> AASGSALIFDEEMSRYKLLWTDPACEIEVPERLTVSYEALRTHGLAQRCKAVPVRQATEQEILLAHSEEYLEAVKQTPGMNVEELMAFSKKYNDVYFHQNIYHCAKLAAGATLQLVDSVMKREVRNGMALVRPPGHHSQRSAANGFCVFNNVAFAALYAKKNYNLNRILIVDWDVHHGQGIQYCFEEDPSVLYFSWHRYEHQSFWPNLPESDYSSVGKGKGSGFNINLPWNKVGMTNSDYLAAFFHVLLPVAYEFDPELVIVSAGFDSAIGDPEGEMCALPEIFAHLTHLLMPLAAGKMCVVLEGGFNLTSLGQSVCQTVHSLLGDPTPRISGLGTACDSALESIQNVRNVQSSYWSSFKHLAQSETNPKRPRLDATNGGPKESSEPASESNPKKTAQDIVWPEPLKRMPASVRTVVVPPPGVELTLPKNCQHSGDISESTAKEVQRIRDKHFHDLTDQNILRSLGNIISVLDRMMRS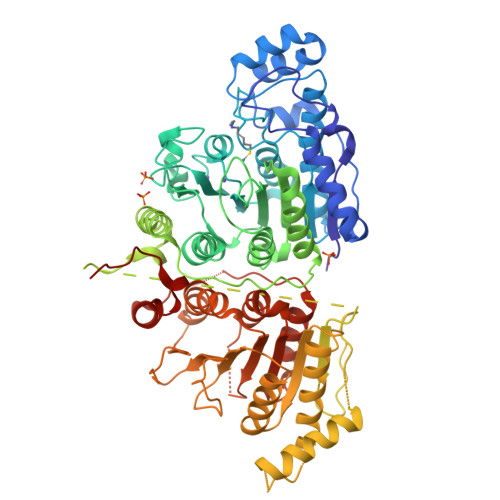DEVCNGCVVVSDLSVSVQCALQHALTEPAERVLVVYVGDGELPVKTNDGKVFLVQICTKETEDKCVNRLTLCLREGESLTAGFMQALLGLILPVAYEFNPALVLGIVEETAAKTRLMRVWGHMTCLIQGLARGRMLTLLQGYDKDLLELTVSALSGASISPLGPLRAPKPEDVEMMEKQRQRLQERWGLLRCTVSESW> MNKESKDDDMSLGKFSFSHFLYYLVLIVVIVYGLYKLFTGHGSDINFGKFLLRTSPYMWANLGIALCVG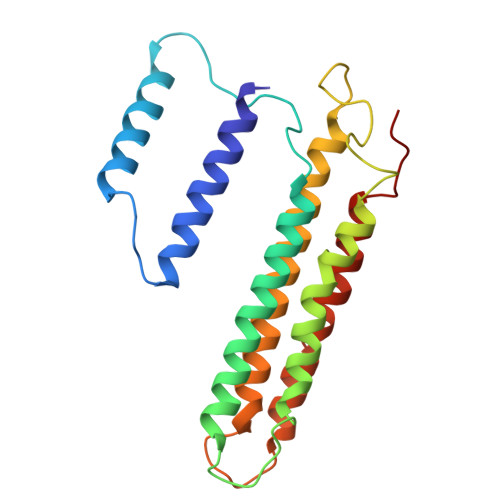LSVVGAAWGIFITGSSMIGAGVRAPRITTKNLISIIFCEVVAIYGLIIAIVFSSKLTVATAENMYSKSNLYTGYSLFWAGITVGASNLICGIAVGITGATAAISDAADSALFVKILVIEIFGSILGLLGLIVGLLMAGKASEFQ> LPTSNPAQ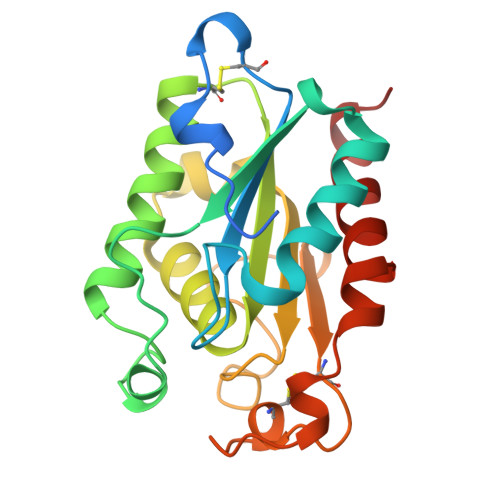ELEARQLGRTTRDDLINGNSASCADVIFIYARGSTETGNLGTLGPSIASNLESAFGKDGVWIQGVGGAYRATLGDNALPRGTSSAAIREMLGLFQQANTKCPDATYIAGGYSQGAALAAASIEDLDSAIRDKIAGTVLFGYTKNLQNRGRIPNYPADRTKVFCNTGDLVCTGSLIVAAPHLAYGPDARGPAPEFLIEKVRAVRGSA>MKYQVLTVGNPNSGKTTLFNGLTGAKQQVGNWAGVTVEKKTGSFVHAGDEFSLTDLPGIYALDSGNDSNSIDESIASRAVLTHPADVIINVVDATCLERSLYMTLQLRELRRPMIVVLNKMDALKRERVHLDLKQLEAFLGCPVLALSANNKEQVRRFKEKLHKLLVQGIALKQIELHYGAEFESLIHELEPMFAEQAVSARALAIRALENDRLVINGLKEAERQNVEQRQHECQVDIDLLVANVRYTYLHELCTHVRRTEGKLSHKFTEKAKLAAALEHHHHHH[4x]

For this bacterium, Feo is the primary system that transports Fe2+ into the cytosol. FeoA and FeoC are known to be small (ca. 7–10 kDa) cytosolic proteins, while FeoB is a large (ca. 80–100 kDa) polytopic transmembrane protein that contains an N-terminal soluble G-protein-like domain termed NFeoB. The status of GTP and GDP bound to the NFeoB region is hypothesized to control the opening and closing of the FeoB pore and therefore the translocation of Fe2+ into the bacterial cytosol.

Despite extensive fine screening and testing of multiple conditions, we were only able to generate datasets of GDP-bound VcNFeoB(His)6 that diffracted modestly, but completely, to 4.2 Å resolution in the C121 space group consistent with 4 molecules in the asymmetric unit (ASU). Using molecular replacement with our 2.3 Å apo VcNFeoB structure coupled with strongly restrained refinement approaches, we built a model that clearly displayed GDP in the nucleotide-binding pocket of all molecules in the ASU based on omit maps. The crystal structure of VcNFeoB(His)6 bound to GDP reveals multiple amino acids that contribute to nucleotide binding. In the absence of nucleotide, the binding pocket is fairly open, while binding of GDP elicits a contraction surrounding the nucleobase with the associated amino acids responsible for nucleotide recognition coming together. In this structure, the Switch I loop that is important for GTP hydrolysis is mostly disordered, which may be attributed to the flexibility of this region when GDP is bound. As the nucleobase enters the binding pocket, a region of random coil from Asn119 to Asp122 tightens, and both residues (conserved amongst NFeoBs) become within hydrogen-bonding distance (3.5 and 2.8 Å, respectively) of the guanine purine. Underneath the guanine purine is Lys120, also conserved in many NFeoBs, which appears to prop up the hydrolyzed nucleotide in the binding pocket; electrostatic contributions from this residue are not observed in our structure, and in some NFeoBs (like those in S. thermophilus, K. pneumoniae, E. coli and Gallionella capsiferriformans, and Thermotoga maritima) this residue corresponds to a non-polar amino acid, either a Met or an Ala. Interestingly, Asn150 is positioned along a region of random coil (known as the G5 motif) above the guanine purine but turned towards, and tightly hydrogen bonded with Asp122 on the G4 motif (2.3 Å distance). While the general NFeoB G-protein-like fold is conserved in our structures, the GDP-bound WT VcNFeoB(His)6 structure revealed interactions between Asn150 (G5 motif) and Asp122 (G4 motif) that caused Asp122 to decrease the number of interactions it makes with the guanine nucleobase.> GEASPVDPLRPVVDASIQPLLKEHRIPGMAVAVLKDGKAHYFNYGVANRESGAGVSEQTLFEIGSVSKTLTATLGAYAVVKGAMQLDDKASRHAPWLKGSAFDSITMGELATYSAGGLPLQFPEEVDSSEKMRAYYRQWAPVYSPGSHRQYSNPSI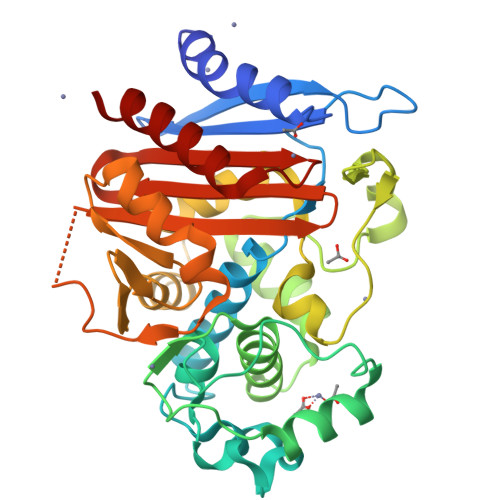GLFGHLAASSLKQPFAPLMEQTLLPGLGMHHTYVNVPKQAMASYAYGYSKEDKPIRVNPGMLADEAYGIKTSSADLLRFVKANIGGVDDKALQQAISLTHQGHYSVGGMTQGLGWESYAYPVTEQTLLAGNSAKVILEANPTAAPRESGSQVLFNKTGSTNGFGAYVAFVPARGIGIVMLANRNYPIEARIKAAHAILAQLAG>MGVNDLWQILEPVKQHIPLRNLGGKTIAVNLSLWVCEAQTVKKMMGSVMKPHLRNLFFRISYLTQMDVKLVFVMEGEPPKLKADVISKRNQTRYGSSGKSWSQKTGRSHFKSVLRECLHMLECLGIPWVQAAGEAEAMCAYLNAGGHVDGCLTNDGDTFLYGAQTVYRNFTMNTKDPHVDCYTMSSIKSKLGLDRDALVGLAILLGCDYLPKGVPGVGKEQALKLIQILKGQSLLQRFNRWNETSCNSSPQLLVTKKLAHCSVCSHPGSPKDHERNGCRLCKSDKYCEPHDYEYCCPCEWHRTEHDRQLNEVENNIKKKACCCEGFPFHEVIQEFLLNKDKLVKVIRYQRPDLLLFQRFTLEKMEWPNHYACEKLLVLLTHYDMIERKLGSRNSNQLQPIRIVKTRIRNGVHCFEIEWEKPEHYAMEDKQHGEFALLTIEEESLFEAAYPEIVAVYQ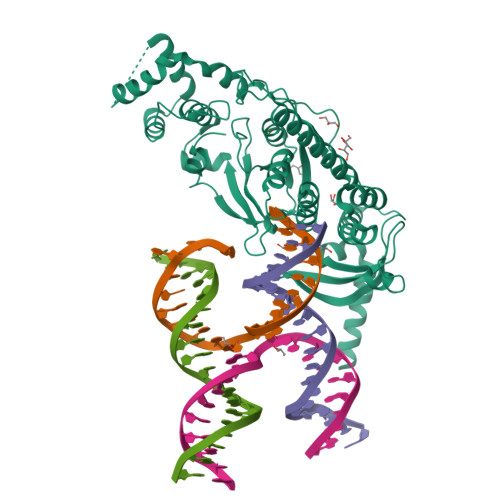KQKLEIKGKKQKRIKPKENNLPEPDEVMSFQSHMTLKPTCEIFHKQNSL[2x]> GAACGACACTGA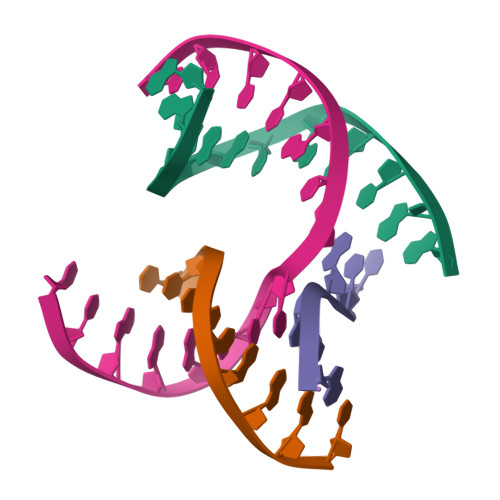;> CGGAGACTC;> TCACCG;> TCGAGTCTGTGTCGT> HHHHHHDDDDKVRSVNFDPDAWEDFLFWLAADRKTARRITRLIGEIQRDPFSGIGKPEPLQGELSGYWSRRIDDEHRLVYRAG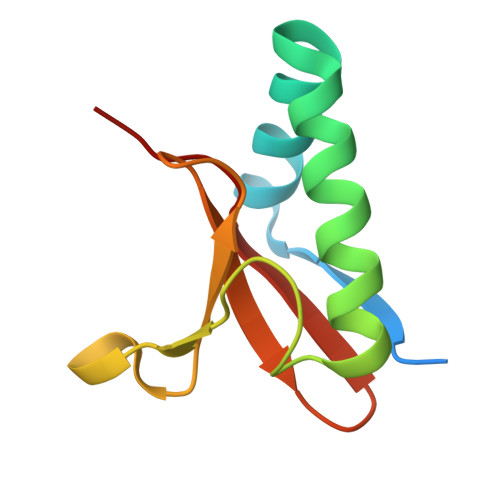DDEVTMLKARYHY>[4x]GAMGMDEGDGEGNI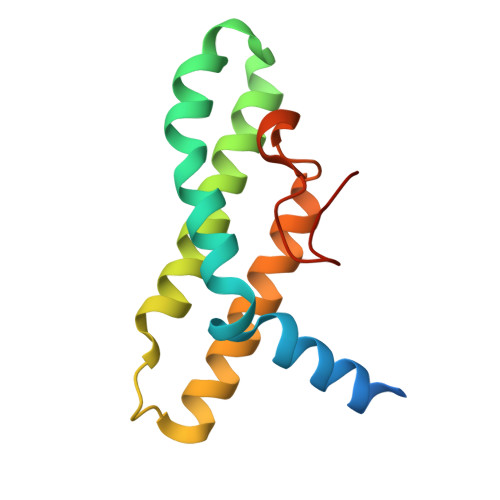LPIMQSIMQNLLSKDVLYPSLKEITEKYPEWLQSHRESLPPEQFEKYQEQHSVMCKICEQFEAETPTDSETTQKARFEMVLDLMQQLQDLGHPPKELAGEMPPGLNFDLDAL> MASYGQTCPRPMCIPPSYADLGKAARDIFNKGFGFGLVKLDVKTKSCSGVEFSTSGSSNTDTGKVTGTLETKYKWCEYGLTFTEKWNTDNTLGTEIAIEDQICQGLKLTFDTTFSPNTGKKSGKIKSSYKRECVNLGCDVD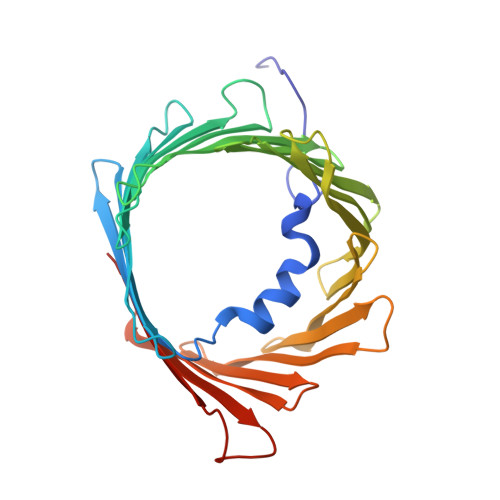FDFAGPAIHGSAVFGYEGWLAGYQMTFDSAKSKLTRNNFAVGYRTGDFQLHTNVNDGTEFGGSIYQKVCEDLDTSVNLAWTSGTNCTRFGIAAKYQLDPTASISAKVNNSSLIGVGYTQTLRPGVKLTLSALVDGKSINAGGHKLGLALELEA> ANENILKLKLYRSLGVILDLENDQVLINRKNDGNIDILPLDNNLSDFYKTKYIWERLGK;> SNANDAAEVALYERLLQLRVLPGASDVHDVRFVF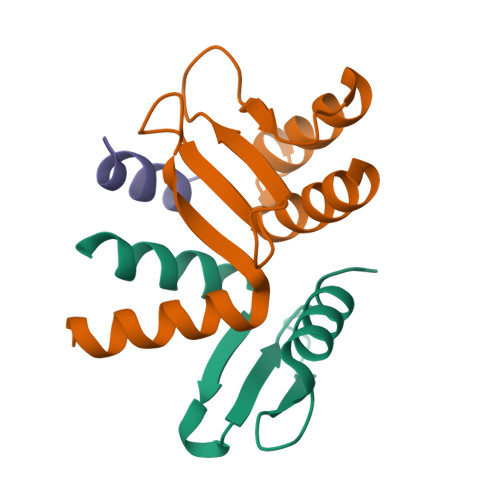GDDSRCWIEVAMHGDHVIGNSHPALDPKSRATLEHVLTVQGDLAAFLVVARDMLLASL;> QQLLKGLSLSFSK> GAMGSMSKSLKKLVEESREKNQPEVDMSDRGISNMLDVNGLFTLSHITQLVLSHNKLTMVPPNIAELKNLEVLNFFNNQIEELPTQISSLQKLKHLNLGMNRLNTLP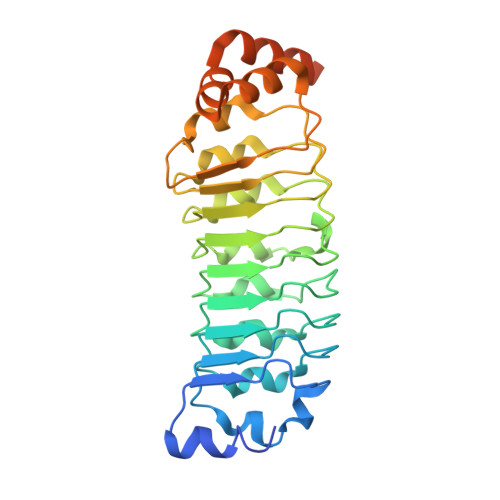RGFGSLPALEVLDLTYNNLSENSLPGNFFYLTTLRALYLSDNDFEILPPDIGKLTKLQILSLRDNDLISLPKEIGELTQLKELHIQGNRLTVLPPELGNLDLTGQKQVFKAENNPWVTPIADQFQLGVSHVFEYIRSETYKYLYGRHMQANPEPPKKNNDKSKKISRKPLAAKNR>MPKPYVAINMVEVRNDPKTLELFGKVGPKVCMVTARHPGFVGFQNHVQIGVVPLGTRWGGAKMEMSQEMHSLMLMQYTFWKNWKDHEEMHKQNWANLFRLCLQCADQMIWGPYEPLYEIVYANMPLNTEMTDFTVMVGKKFAAGEAVSIPPISQPYGKRVVAFGEHIVKEGLENQFEEYAIKTLEAFRSAPGFLGGMILKEIGVSPLGSLQLNAKGFHQILETANGMDVPEPVTIYEAPEFRNRPQRYIVHTEWSDTNALMFGLGRVLIYPEVRQIHDKVLDTLVYGPYIRVLNPMMEGT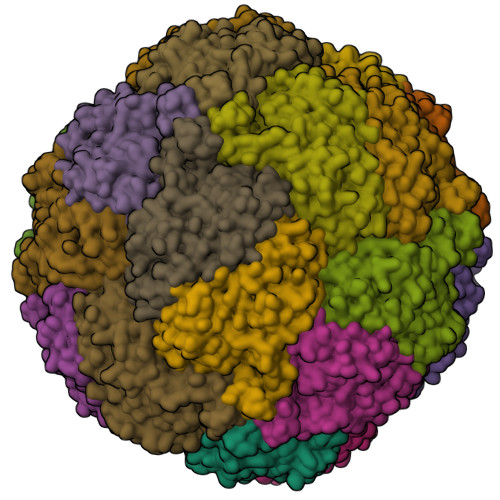YWREYLNEYHL[24x]> GSHMVPAALPQLTPTLVSLLEVIEPEVLYAGYDSSVPDSAWRIMTTLNMLGGRQVIAAVKWAKAIPGFRNLHLDDQMTLLQYSWMSLMVFALGWRSYRQASGNLLCFAPDLIINEQRMTLPCMYDQCKHMLFISTELQRLQVSYEEYLCMKTLLLLSSVPKEGLKSQELFDEIRMTYIKELG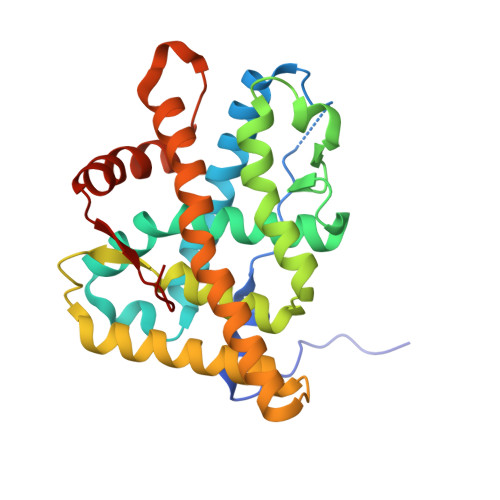KAIVKREGNSSQNWQRFYQLTKLLDSMHDVVENLLSYCFQTFLDKSMSIEFPEMLAEIITNQIPKYSNGNIKKLLFHQK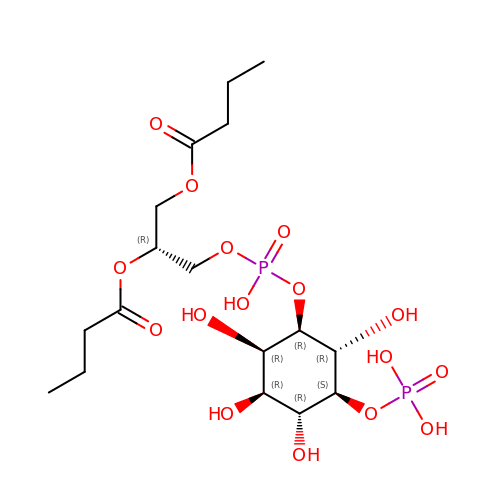(2R)-3-{[(S)-hydroxy{[(1R,2R,3R,4R,5S,6R)-2,3,4,6-tetrahydroxy-5-(phosphonooxy)cyclohexyl]oxy}phosphoryl]oxy}propane-1,2-diyl dibutanoate | C17 H32 O16 P2 | NKJZZWLREOAJGO-FBVWBLDGSA-N>DYFQGAMGSKPAYSFHVTADGQMQPVPFPPDALIGPGIPRHARQINTLNHGEVVCAVTISNPTRHVYTGGKGCVKVWDISHPGNKSPVSQLDCLNRDNYIRSCKLLPDGCTLIVGGEASTLSIWDLAAPTPRIKAELTSSAPACYALAISPDSKVCFSCCSDGNIAVWDLHNQTLVRQFQGHTDGASCIDISNDGTKLWTGGL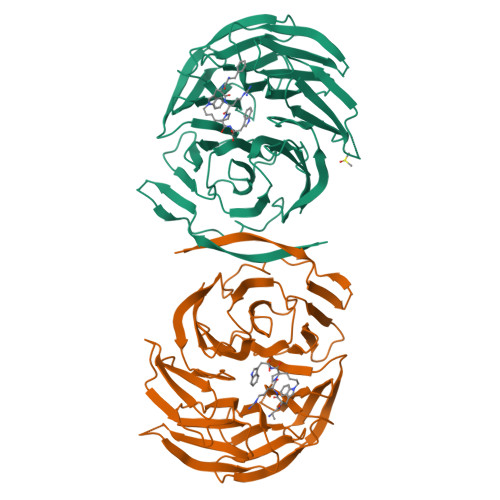DNTVRSWDLREGRQLQQHDFTSQIFSLGYCPTGEWLAVGMESSNVEVLHVNKPDKYQLHLHESCVLSLKFAYCGKWFVSTGKDNLLNAWRTPYGASIFQSKESSSVLSCDISVDDKYIVTGSGDKKATVYEVIY[2x]>[2x]GPGSMSDQSSQHFIHARQALLPDGWAENVRIGIAGGVICSIETGVLAGPDDERQSVVVAGMANLHSHAFQYGMAGLAERRGPSADSFWSWREIMYKFALTMTPEQAEAVALRLYVDMLEAGFTRVGEFHYLHHDCDGTPYANLSEMADRIAAAATTAGMGLTLLPVFYAHSGFGGAAANEGQRRFINDPERFARLIEGCRKTLEGFEGAVLGVAPHSLRAVTP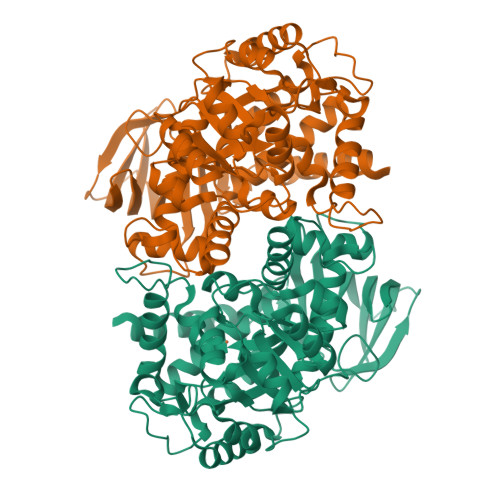DELDSVTQLLPDAPVHIHVAEQVKEVEDCIAWSGKRPVEWLLDHQDVTARWCLIHATHMSDEETKHMAKAGAIAGLCPVTEANLGDGTFNATEFAAAGGKFGIGSDSNVLIGIGDELRQLEYSQRLYHRARNVLAANEGSTGRALFDGAVLGGNIAMGRPEDGLKKGASADFVSLDVERLPHAKGDVVLDGWIFAGRAHVCDVWVRGVKQVEGGRHRLRDEAERAFQKALGELLA5-chloranyl-N2-[(1S)-1-(5-fluoranylpyridin-2-yl)ethyl]-N4-(3-propan-2-yloxy-1H-pyrazol-5-yl)pyrimidine-2,4-diamine | C17 H19 Cl F N7 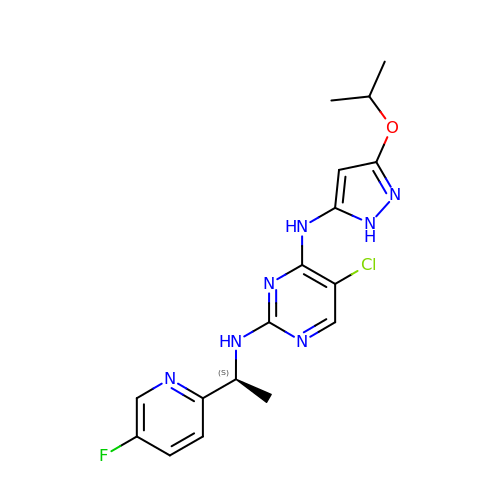O | LBVKEEFIPBQIMD-JTQLQIEISA-N> GHMLWARLVGLARLEARALSKKERRSLL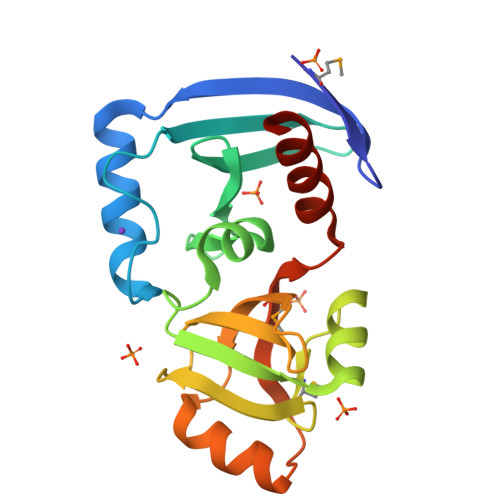ERLKPYYTRIPFSEKADLRLVKARTDSGEYEIITVDGVPCLFEWSDGRIYPTLQCLKAFGVDWLKGVVLVDKGAAIALAKGAHLMIPGVVGVEGSFTRGDVVAALYHETRTPVMVGVAEVDSSALEKLYREKARGRAVRRVHRLGDALWELAQEVGKRLSGS>[6x]MGSSHHHHHHSSGLVPAGSHSKVFIRSAINRVHQNSAANGGELPRIVFPEGTSTKVLKALATLVEEKICQPILLGYPERVKEKIKALDIPLLNDVSIVHPSSHPKYFSFVEKLYSLAQRKGINLGEAERLMADPNYFAAMMVNQGEADGMVSGSSINYADAVRPILQTIGVYKEGIPAGLNFVLLEDKFLVLADTTVNLNPTAEQCAQIALQAAKIVEYFGIEPRVAMLSYSNFSGAEGTPRKMKKAAEIARSLRPDLMIEGDMQADTAVNPEIMERLFPFSGLKGGANVLVFPNLESSNIAYKLIQQIGKAEVIGPFLTGVRRSANVLQRTTTVDGIVNSVVFTALEAQYIKEVLKSRGKK

Bacterial hybrid malic enzymes (MaeB grouping, multidomain) catalyse the transformation of malate to pyruvate, and are a major contributor to cellular reducing power and carbon flux. Distinct from other malic enzyme subtypes, the hybrid enzymes are regulated by acetyl-CoA, a molecular indicator of the metabolic state of the cell. The larger ME isoforms (hybrid enzymes) are predicted to be a fusion of two unrelated enzymes; a catalytic N-terminal ME subunit and a C-terminal phosphotransacetylase (PTA) domain. The PTA domain is homologous to PTA enzymes (that interconvert acetyl-CoA and phosphate to CoA and acetyl phosphate), yet they appear to lack critical catalytic residues and thus acts as a sensor instead.

An extension from d1 (residues 524–550, forming a loop with two helices that we term the 3′ loop) sits over the 3′-phosphate group, interacting via residues R535 and K538. Using HPLC as a readout, we were able to prevent acetyl-CoA binding by mutating R535 that makes a direct contact to the 3′ phosphate group. Variants R535E and R535A abolished acetyl-CoA binding, and generated an enzyme insensitive to allosteric inhibition by both CoA and acetyl-CoA, although these mutants retained ~70% activity to wild-type (wt) MaeB. We were also able to generate structures for R535E, R535A and N718D PTA domain variants, which demonstrate the same features as the wt PTAapo structure.>MSQTHKHAIPANIADRCLINPEQYETKYKQSINDPDTFWGEQGKILDWITPYQKVKNTSFAPGNVSIKWYEDGTLNLAANCLDRHLQENGDRTAIIWEGDDTSQSKHISYRELHRDVCRFANTLLDLGIKKGDVVAIYMPMVPEAAVAMLACARIGAVHSVIFGGFSPEAVAGRIIDSSSRLVITADEGVRAGASIPLKKNVDDALKNPNVTSVEHVIVLKRTGSDIDWQEGRDLWWRDLIEKASPEHQPEAMNAEDPLFILYTSGSTGKPKGVLHTTGGYLVYAATTFKYVFDYHPGDIYWCTADVGWVTGHSYLLYGPLACGATTLMFEGVPNWPTPARMCQVVDKHQVNILYTAPTAIRALMAEGDKAIEGTDRSSLRILGSVGEPINPEAWEWYWKKIGKEKCPVVDTWWQTETGGFMITPLPGAIELKAGSATRPFFGVQPALVDNEGHPQEGATEGNLVITDSWPGQARTLFGDHERFEQTYFSTFKNM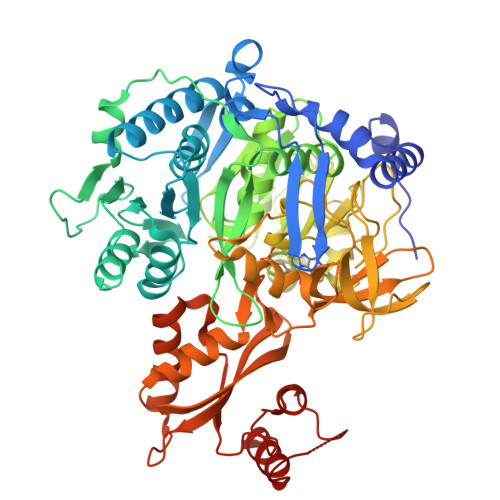YFSGDGARRDEDGYYWITGRVDDVLNVSGHRLGTAEIESALVAHPKIAEAAVVGIPHAIKGQAIYAYVTLNHGEEPSPELYAEVRNWVRKEIGPLATPDVLHWTDSLPKTRSGKIMRRILRKIAAGDTSNLGDTSTLADPGVVEKLLEEKQAIAMPS[2x]>[6x]MNDVEKLVKLLTSTDSETQKEAARDLAEIASGPASAIKAIVDAGGVEVLVKLLTSTDSEVQKEAARALANIASGPDEAIKAIVDAGGVEVLVKLLTSTDSEVQKEAARALANIASGPDEAIKAIVD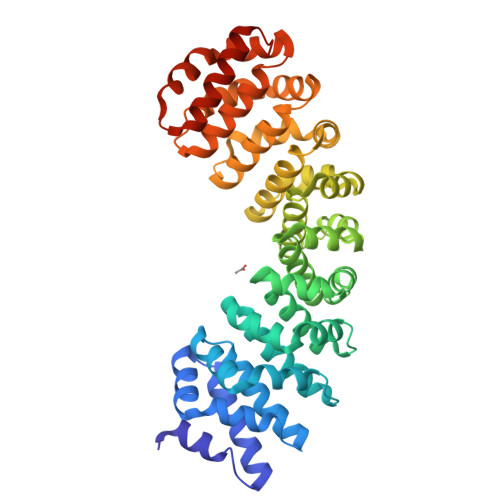AGGVEVLVKLLTSTDSEVQKEAARALANIASGPDEAIKAIVDAGGVEVLVKLLTSTDSEVQKEAARALANIASGPTSAIKAIVDAGGVEVLVKLLTSTDSEVQKEAARALANIASGPDEAIKAIVDAGGVEVLVKLLTSTDSEVQKEAARALANIASGPDEAIKAIVDAGGVEVLVKLLTSTDSEVQKEAARALANIASGPDEAIKAIVDAGGVEVLVKLLTSTDSEVQKEAARALANIASGPTSAIKAIVDAGGVEVLQKLLTSTDSEVQKEAQRALENIKSGGWLEHHHHHH> MGSSHHHHHHSSGLVPRGSAADLDTQRSDIATLLKTSLRKGDTWYLVDSRWFKQWKKYVGFDSWDKYQMGDQNVYPGPIDNSGLLKDGDAQSLKEHLIDELDYILLPTEGWNKLVSWYTLMEGQEPIARKVVEQGMFVKHCKVEVYLTELKLCENGNMNNVVTRRFSKADTIDTIEKEIRKIFSIPDEKETRLWNKYMSNTFEP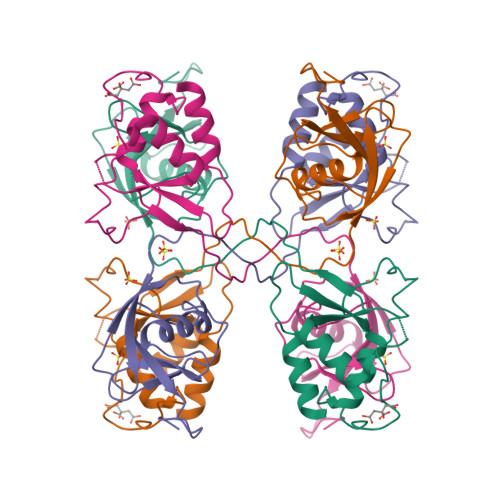LNKPDSTIQDAGLYQGQVLVIEQKNEDGTWPRG> GSMSSRKKVLLKVIILGDSGVGKTSLMNQYVNKKFSASYKATIGADFLTREVMVDDRQVTMQLWDTAGQERFQSLGVAFYRGADCCVLVFDV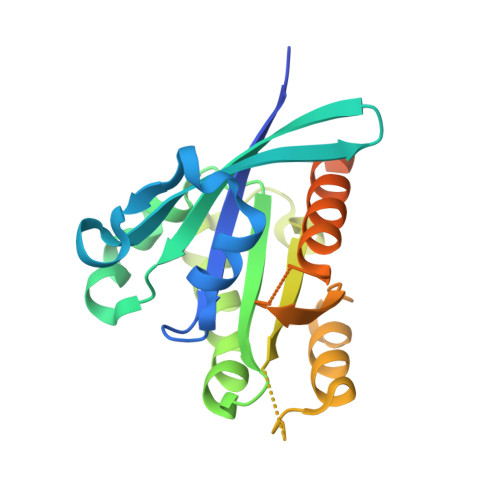NNAKSFDALDSWRDEFLIQASPRDPENFPFVVLGIKIDVEESKRVISTKRAQTFCQSKGGIPYFETSAKEAINVEEAFQVIARNALMQEESEEFSGDFQDPINIHIENERDGCAC>MHHHHHHTSKIEQPRWASKDSAAGAASTPDEKIVLEFMDALTSNDAAKLIEYFAEDTMFQAMPLPPAYGRDAVEQTLAGLFTVMSIDAVETFHIGSSNGLVYTERVDVLRALPTGKSYNLSVLGVFQLTEG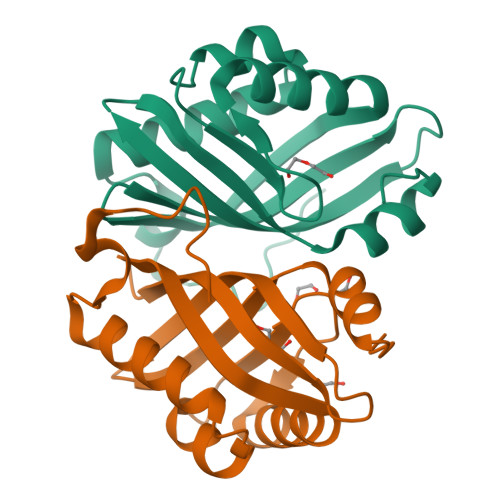KITGWRDYFDLREFEEAVDLPLRG[4x]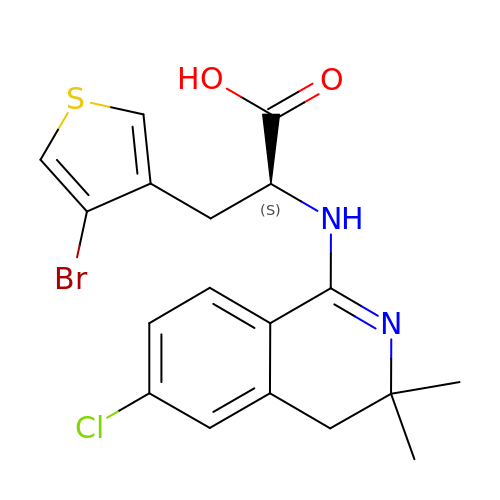3-(4-bromothiophen-3-yl)-N-(6-chloro-3,3-dimethyl-3,4-dihydroisoquinolin-1-yl)-L-alanine | C18 H18 Br Cl N2 O2 S | LZMNPXMCRBRYAN-HNNXBMFYSA-N>[3x]MRGSHHHHHHRSPSKVQELSVYEINELDRHSPKILKNAFSLMFGLGDLVPFTNKLYTGDLKKRVGITAGLCVVIE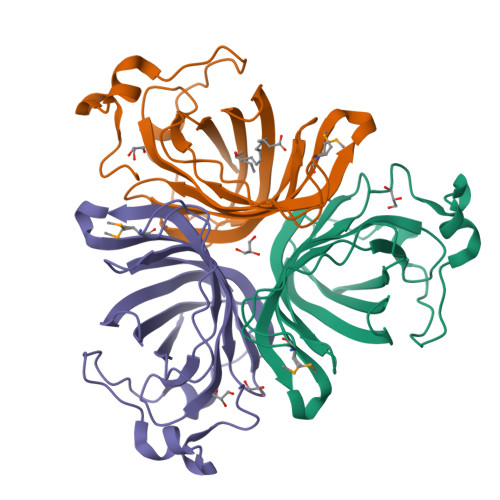HVPEKKGERFEATYSFYFGDYGHLSVQGPYLTYEDSFLAITGGAGIFEGAYGQVKLQQLVYPTKLFYTFYLKGLANDLPLELTGTPVPPSKDIEPAPEAKALEPSGVISNYTN> EQRITLKDYAMRFGQTKTAKDLGVYQSAINKA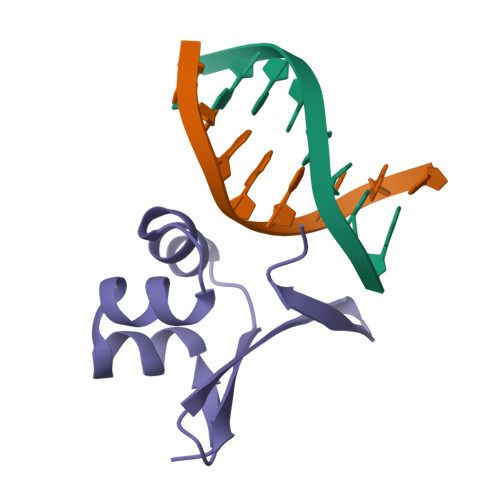IHAGRKIFLTINADGSVYAEEVKDGEVKPFPSN>[6x]MTERTLVLIKPDGIERQLIGEIISRIERKGLTIAALQLRTVSAELASQHYAEHEGKPFFGSLLE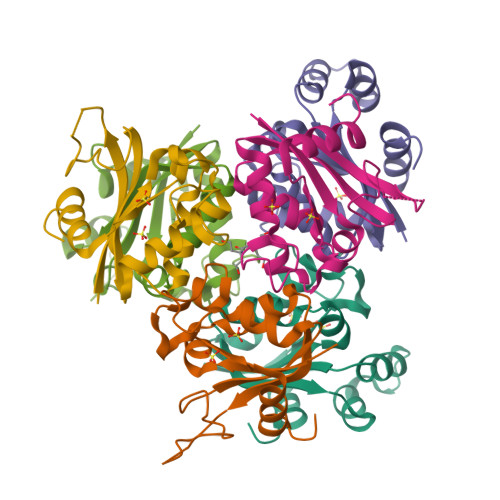FITSGPVVAAIVEGTAAIAAVRQLAGGTDPVQAAAPGTIRGDFALETQFNLVHGSDSAESAQREIALWFPGA> TDYTKYVNTFIGAADNGHTFPGACRPFGMIQTSPVTGAVGWRYCSEYVNSDSIIWGFTQTHLNGTGCMDLGDVLVMPVTGTRTRAWDAYRSRFSKKLEAATPGYYTVELTEPNVKAELTATPHAALHRYTYHNADSASVLIDLQHGPTWNENQYHSQVKECEVNWEDAQTLTGHVRNSVWVNQDYFFVMKFNRPVTDSLYLPMGETEKGKRIIASFDMQPGEELLMKVALSTTGIEGARKNMEAEVPAWDFEGVKKTAHDDWNSYLSRIDVTGTEDEKTNFYTCFYHALIQPNQISDVDGLYRNAADSVVKAGTGTFYSTFSLWDTYRAAHPFYTLMVPEKVDGFVNSLVEQSEVQGFLPIWGLWGKETYTMVGNHGVSVIAEAYRKGFRGFDAERAFNAIKQTQTVSHKQKSDWETYMKYGYFPTDLIKTESVSSSLESVYDDYAAADMAKRMGKTEDAAYFSKRADFYKNLFDTETQFMRPRNSNGTWKTPFNPSQVAHAESTGGDYTEGNAWQYTWHVQHDVPGLISLFGGEEPFLNKLDSLFTLKLETTQADVTGLIGQYAHGNEPSHHITYLYALAGRPERTQELVREIFDTQYHPEPDGLCGNDDCGQMSAWYMFSAMGFYPVDPVSGNYVFGAPQMPKIVLHLADGKTFTVIADGISKEHKYIDSITLNGEPYTKNYISHEDILKGGTLVYKMKLEHHHHHH

Here we used a functional analysis approach, coupled to detailed biochemistry and structural biology, to reveal a pathway for the degradation of plant N-glycans encoded by the human gut microbiota. We describe the biochemical characterization of five CAZymes and two crystal structures to provide a degradation pathway for plant complex N-glycans encoded by the human gut microbiome. In this study we characterize the likely pathway for the degradation of plant N-glycans by a prominent member of the human gut microbiota. B035DRAFT_03340GH92 is then able to remove the α1,3-mannose, followed by B035DRAFT_00995GH3 to cleave the plant-specific β1,2-xylose, and B035DRAFT_02132GH29 to release the core α1,3-fucose, leaving a Manα1,6Manβ1,4GlcNacβ1,4GlcNac tetrasaccharide.

To investigate the structural basis for the unusual specificity displayed by B035DRAFT_03340GH92 we determined the crystal structure of the enzyme to 1.43 Å. The GH92 consists of two domains: an N-terminal β-sandwich domain composed of 16 antiparallel β-strands domain and an (α/α)6-barrel catalytic domain. These two domains are pinned together by two α-helices, previously dubbed helix 1 and 2. The density for several metal ions was observed bound to the protein surface, which were modeled as Na from the crystallization conditions, except for a Ca near the active site, as this metal has been shown to be key for GH92 activity. The active site of B035DRAFT_03340GH92 is comprised of residues originating from both the N- and C-terminal domains, which is a common feature of the other GH92 structures. The +1 mannose is likely recognized by the side chains of at least three residues: H530, S533, and E532, which are positioned underneath the mannose. Overhanging this subsite (and possibly the +2 GlcNAc position also) are three hydrophobic residues Y72, W178, and W209, which is suggestive of π-stacking of the sugars. The +1 subsite interactions allows space either side of the +1 mannose for the +1″ mannose and +1′ xylose. There are clear pockets for these sugars in the B035DRAFT_03340GH92 structure. The lack of activity seen for BT3991GH92 is likely due to the plant-specific β1,2-xylose on the core mannose causing steric hindrance within the active site, whereas B035DRAFT_03340GH92 is able to accommodate this decoration.>TQTLPAEGEIGLIDVGSLQLESGAVIDDVCIAVQRWGKLSPARDNVVVVLHALTGDSHITGPAGPGHPTPGWWDGVAGPGAPIDTTRWCAVATNVLGGCRGSTGPSSLARDGKPWGSRFPLISIRDQVQADVAALAALGITEVAAVVGGSMGGARALEWVVGYPDRVRAGLLLAVGARATADQIGTQTTQIAAIKADPDWQSGDYHETGRAPDAGLRLARRFAHLTYRGEIELDTRFANHNQGNEDPTAGGRYAVQSYLEHQGDKLLSRFDAGSYVILTEALNSHDVGRGRGGV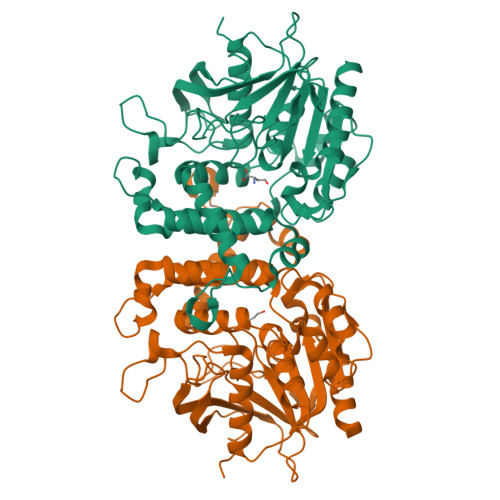SAALRACPVPVVVGGITSDRLYPLRLQQELADLLPGCAGLRVVESVYGHDGFLVETEAVGELIRQTLGLADREG[12x]>[2x]MRSRRVDVMDVMNRLILAMDLMNRDDALRVTGEVR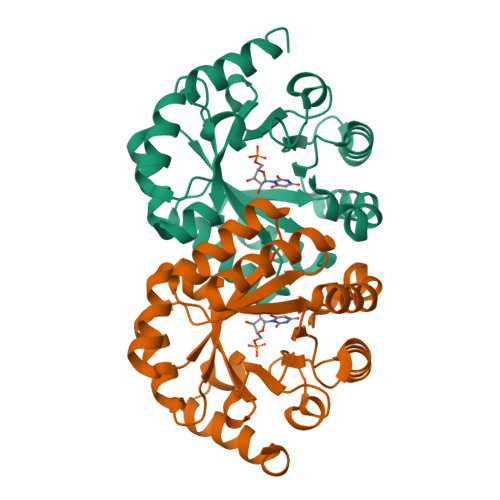EYIDTVKIGYPLVLSEGMDIIAEFRKRFGCRIIADFKVADIPETNEKICRATFKAGADAIIVHGFPGADSVRACLNVAEEMGREVFLLTEMSHPGAEMFIQGAADEIARMGVDLGVKNYVGPSVRPERLSRLREIIGQDSFLISPGVGAQGGDPGETLRFADAIIVGRSIYLADNPAAAAAGIIESIKDLLNP> AFTQAPMLEQNKQLPPVDQRLPEKPLVIKPIASNGVYGGTLRTVMRGNADGNGILRTIGPQGLTHWTQDIQTVEPYVAESYTVSPDAMEYTFKLRKGMKWSDGTPFTADDIVFAMNDVVLNKEMFPQTPSAYLVGGKAPKVSKVDDYTVKFEFPAANLSFPETLATPLGQHPTLYQKKYCSQFHPAYNKNVQAEFTKANVKDWPSLMRAKCSDIELPSRWSSTERPSIDPWLIKEPYGGAVTRVVMERNPFYWQVDPTGKQLPYVDRIQYAVVSDLQAIILAATNGQYDIEARLLGSDVTSRPLMLKNQ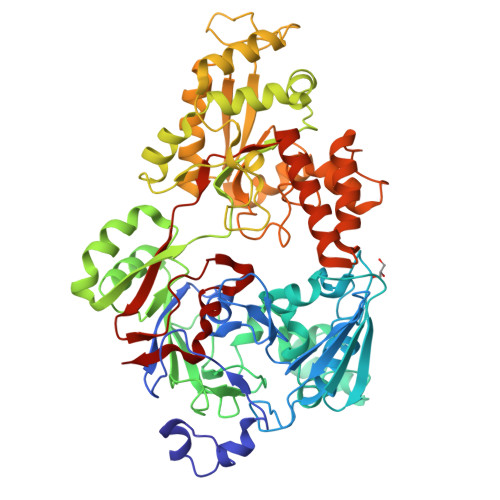QKGGYKVFGQTSANANAAGLWLNQTTKNEKLRKYMTQHDFRQALSLAMDRDEINKVAWLGQAAPWQSGPFKESKWYNEKLATQYLKLDLAQANQILDRLGLTKRDSDGYRTYPDGGRVSLDAIVMIDRQAMVQTLELIRRQWQKAGVELVIKGSERSLFYNRATANDYDISIDVFPGGLDATLNPRAYVAVHPLESRMSLEWAKWYLSGGKQGIEPNESMKKRMALYDQFVAAKTQSQALSLFKQILQISADEFEVIGTVRPAVISSLHSLKLQNVNEKMPFGWPYATPSLSLPQQWYFS>[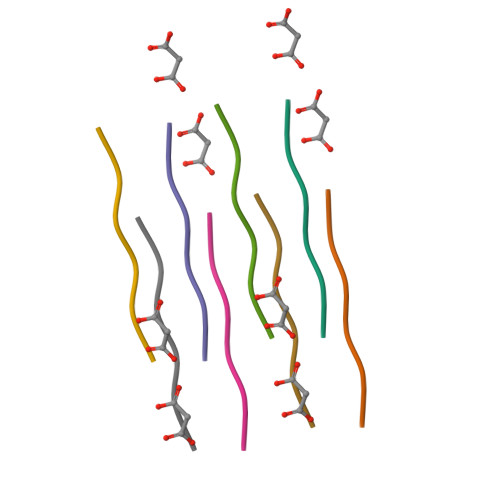2x]AGAAAA> MSFESKKPMRTWSHLAEMRKKPSEYDIVSRKLHYSTNNPDSPWELSPDSPMNLWYKQYRNASPLKHDNWDAFTDPDQLVYRTYNLMQDGQESYVQSLFDQFNEREHDQMVREGWEHTMARCYSPLRYLFHCLQMSSAYVQQMAPASTISNCCILQTADSLRWLTHTAYRTHELSLTYPDAGLGEHERELWEKEPGWQGLRELMEKQLTAFDWGEAFV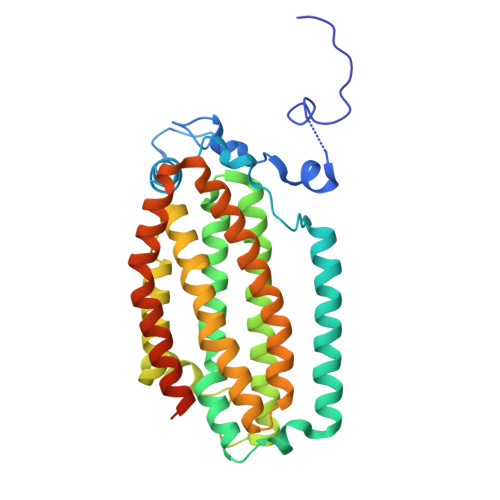SLNLVVKPMIVESIFKPLQQQAWENNDTLLPLLIDSQLKDAERHSRWSKALVKHALENPDNHAVIEGWIEKWRPLADRAAEAYLSMLSSDILHAQYLERSTSLRASILTV3-(7-HYDROXY-8-RIBITYLLUMAZINE-6-YL) PROPIONIC ACID | C14 H18 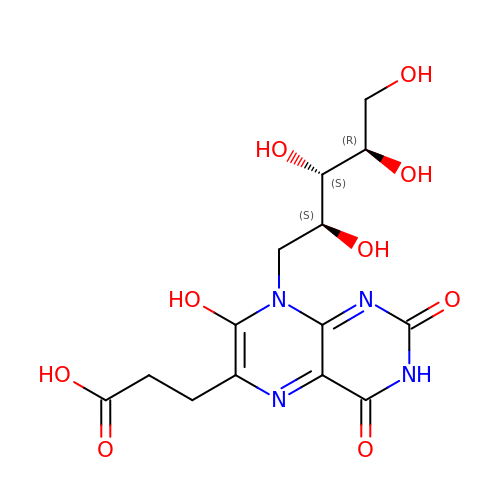N4 O9 | ZUXCIPRCLKZSHS-PJKMHFRUSA-N>QIFNFSSGPAMLPAEVLKQAQQELRDWNGLGTSVMEVSHRGKEFIQVAEEAEKDFRDLLNVPSNYKVLFCHGGGRGQFAAVPLNILGDKTTADYVDAGYWAASAIKEAKKYCTPNVFDAKVTVDGLRAVKPMREWQLSDNAAYMHYCPNETIDGIAIDETPDFGADVVVAADFSSTILSRPIDVSRYGVIYAGAQKNIGPAGLTIVIVREDLLGKANIACPSILDYSILNDNGSMFNTPPTFAWYLSGLVFKWLKANGGVAEMDKINQQKAELLYGVIDNSDFYRNDVAKRNRSRM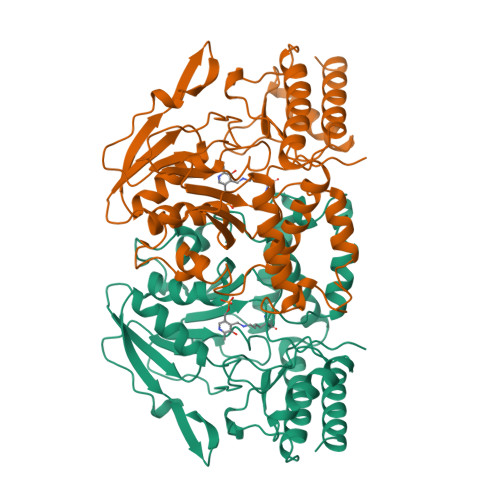NVPFQLADSALDKLFLEESFAAGLHALKGHRVVGGMRASIYNAMPLEGVKALTDFMVEFERRHG[2x]> MSAKAISEQTGKELLYKFICTTSAIQNRFKYARVTPDTDWARLLQDHPWLLSQNLVVKPDQLIKRRGKLGLVGVNLTLDGVKSWLKPRLGQEATVGKATGFLKNFLIEPFVPHSQAEEFYVCIYATREGDYVLFHHEGGVDVGDVDAKAQKLLVGVDEKLNPEDIKKHLLVHAPEDKKEILASFISGLFNFYEDLYFTYLEINPLVVTKDGVYVLDLAAKVDATADYICKVKWGDIEFPPPFGREAYPEEAYIADLDAKSGASLKLTLLNPKGRIWTMVAGGGASVVYSDTICDLGGVNELANYGEYSGAPSEQQTYDYAKTILSLMTREKHPDGKILIIGGSIANFTNVAATFKGIVRAIRDYQGPLKEHEVTIFVRRGGPNYQEGLRVMGEVGKTTGIPIHVFGTETHMT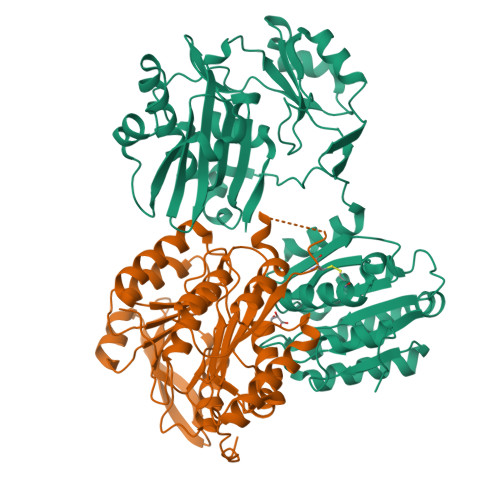AIVGMALGHRPIP;> GKSTTLFSRHTKAIVWGMQTRAVQGMLDFDYVCSRDEPSVAAMVYPFTGDHKQKFYWGHKEILIPVFKNMADAMRKHPEVDVLINFASLRSAYDSTMETMNYAQIRTIAIIAEGIPEALTRKLIKKADQKGVTIIGPATVGGIKPGCFKIGNTGGMLDNILASKLYRPGSVAYVSRSGGMSNELNNIISRTTDGVYEGVAIGGDRYPGSTFMDHVLRYQDTPGVKMIVVLGEIGGTEEYKICRGIKEGRLTKPIVCWCIGTCATMFSSEVQFGHAGACANQASETAVAKNQALKEAGVFVPRSFDELGEIIQSVYEDLVANGVIVPAQEVPPPTV Unlike other chromatin remodelers, INO80 preferentially mobilizes hexasomes, which can form during transcription. Here, we report cryogenic-electron microscopy (cryo-EM) structures of endogenously purified S. cerevisiae INO80 bound to a hexasome and a nucleosome. We group subunits of the INO80 complex into four modules: Rvb module (Rvb1/Rvb2), Arp8 module (Arp8/Arp4/Actin/Ies4 and Taf14), Ino80 module (Ino80/Ies2) and Arp5 module (Arp5/Ies6). The Ino80 protein consists of three major regions: the N-terminal domain (NTD), the HSA region (Ino80HSA) and the ATPase domain (Ino80ATPase).

While the INO80 architecture appears similar to that in the INO80-nucleosome structures, a major difference is that it is rotated ~180° on a hexasome compared to a nucleosome. On a hexasome, INO80 places its ATPase subunit, Ino80, at superhelical location (SHL)-2, across from SHL-6/−7 as previously seen on nucleosomes. When INO80 binds to a hexasome, the Arp5/Ies6 regions used in the context of a nucleosome are repurposed for different interactions. We observe that Ino80ATPase engages the hexasome predominantly near SHL −2. The placement of Ino80ATPase near SHL-2 is consistent with how the ATPase subunits of other remodelers bind the nucleosome. A site-specific gap at SHL-2 substantially inhibits INO80’s sliding of hexasomes (~2000 fold) while a gap near SHL-6 does not have a major effect. We further propose that the new contacts made by the Arp5/Ies6 module with the exposed H3-H4 surface provide an anchor allowing the Ino80 motor to efficiently pump DNA through the hexasome. These findings also explain the differential effects of the Arp5/Ies6 module on hexasome versus nucleosome sliding.

> IEIDVLCDLTQRQAKLYQVLKSQISTNYDAIENAATNDSTSNSASNSGSDQNLINAVMQFRKVCNHPDLFERADVDSPFSFTTFGKTTSMLTASVANNNSSVISNSNMNLSSMSSNNISNGKFTDLIYSSRNPIKYSLPRLIYEDLILPNYNNDVDIANKLKNVKFNIFNPSTNYELCLFLSKLTGEPSLNEFFRVSTTPLLKRVIERTNGPKNTDSLSFKTITQELLEVTRNAPSEGVMASLLNVEKHAYEREYLNCIQRGYHPNVSAPPVTIEVLGSSHVTNSINNELFDPLISQALSDIPAITQYNMHVKKGIPVEDFPKTGLFPEPLNKNFSSNISMPSMDRFITESAKLRKLDELLVKLKSEGHRVLIYFQMTKMMDLMEEYLTYRQYNHIRLDGSSKLEDRRDLVHDWQTNPEIFVFLLSTRAGGLGINLTAADTVIFYDSDWNPTIDSQAMDRAHRLGQTRQVTVYRLLVRGTIEERM;> KAVVIDDPPLRQTPEPFDEQSAYNPQSPIAIDFGSSKLRAGFVNHATPTHIFPNALTKFRDRKLNKNFTFVGNDTLLDQAVRSQSRSPFDGPFVTNWNLTEEILDYTFHHLGVVPDNGIPNPILLTERLATVQSQRTNWYQILFETYNVPGVTFGIDSLFSFYNYNPSGNKTGLVISCGHEDTNVIPVVDGAGILTDAKRINWGGHQAVDYLNDLMALKYPYFPTKMSYLQYETMYKDYCYVSRNYDEDIEKILTLENLDTNDVVVEAPFTEVLQPQKTEEELRIQAEKRKETGKRLQEQARLKRMEKLVQKQEEFEYFSKVRDQLIDEPKKKVLSVLQNAGFDDERDFKKYLHSLEQSLKKAQMVEAEDDSHLDEMNEDKTAQKFDLLDIADEDLNEDQIKEKRKQRFLKASQDARQKAKEEKERVAKEEEEKKLKEQQWRETDLNGWIKDKRLKLNKLIKRRKEKLKLRDEMKDRKSQVSQNRMKNLASLAEDNVKQGAKRNRHQATIDNDPNDTFGANDEDWLIYTDITQNPEAFEEALEYEYKDIVELERLLLEHDPNFTEEDTLEAQYDWRNSILHLFLRGPRPHDSENIHEQHQMHLNVERIRVPEVIFQPTMGGQDQAGICELSETILLKKFGSQPGKLSQTSIDMVNNVLITGGNAKVPGLKERIVKEFTGFLPTGTNITVNMSSDPSLDAWKGMAALARNEEQYRKTVISKKEYEEYGPEYIKEHKLGNTKYFED;> ERLLFLRSVGERNEIGFPSRFKSAHYKKPTRRHKSARQLISDENKRINALLTKANKAAESSTAARRLVPKATYFSVEAPPSIRPAKKYCDVTGLKGFYKSPTNNIRYHNAEIYQLIVKPMAPGVDQEYLKLRGANFVLK;>[3x]VTRTAAHTHIKGLGLDESGVAKRVEGGFVGQIEAREACGVIVDLIKAKKMSGRAILLAGGPSTGKTALALAISQELGPKVPFCPLVGSELYSVEVKKTETLMENFRRAIGLRIKETKEVYEGEVTELTPEDAENPLGGYGKTISHVIVGLKSAKGTKTLRLDPTIYESIQREKVSIGDVIYIEANTGAVKRVGRSDAYATEFDLETEEYVPLPKGEVHKKKEIVQDVTLHDLDVANARPQGGQDVISMMGQLLKPKKTEITEKLRQEVNKVVAKYIDQGVAELIPGVLFIDEVNMLDIEIFTYLNKALESNIAPVVVLASNRGMTTVRGTEDVISPHGVPPDLIDRLLIVRTLPYDKDEIRTIIERRATVERLQVESSALDLLATMGTETSLRYALQLLAPCGILAQTSNRKEIVVNDVNEAKLLFLDAKRSTKILETSANYL;>KSLSLIAAHSHITGLGLDENLQPRPTSEGMVGQLQARRAAGVILKMVQNGTIAGRAVLVAGPPSTGKTALAMGVSQSLGKDVPFTAIAGSEIFSLELSKTEALTQAFRKSIGIKIKEETELIEGEVVEIQIDRSITGGHKQGKLTIKTTDMETIYELGNKMIDGLTKEKVLAGDVISIDKASGKITKLGRSFARSRDYDAMGADTRFVQCPEGELQKRKTVVHTVSLHEIDVINSRTQGFLALFTGDTGEIRSEVRDQINTKVAEWKEEGKAEIVPGVLFIDEVHMLDIECFSFINRALEDEFAPIVMMATNRGVSKTRGTNYKSPHGLPLDLLDRSIIITTKSYNEQEIKTILSIRAQEEEVELSSDALDLLTKTGVETSLRYSSNLISVAQQIAMKRKNNTVEVEDVKRAYLLFLDSARSVKYVQENESQYIDDQGNVQISIAKSADPDAMDTTE[3x];> FVKPRRPYNSEGMTRILRRYEEDLFCTF>[2x]WGAPTITNDGVSIAKEIELEDPYEKIGAELVKEVAKKTDDVAGDGTTTATVLAQALVREGLRNVAAGANPLGLKRGIEKAVEKVTETLLKGAKEVETKEQIAATAAISAGDQSIGDLIAEAMDKVGNEGVITVEESNTFGLQLELTEGMRFDK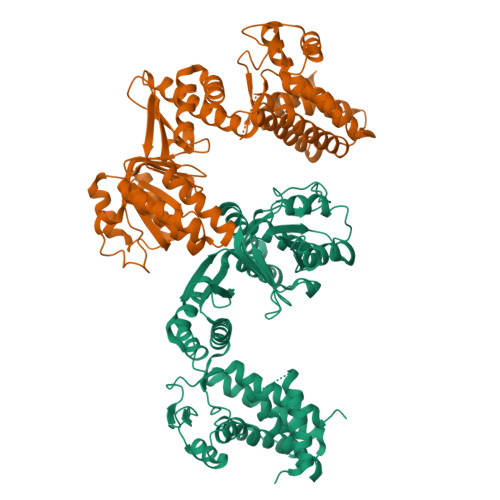GYISGYFVTDPERQEAVLEDPYILLVSSKVSTVKDLLPLLEKVIGAGKPLLIIAEDVEGEALSTLVVNKIRGTFKSVAVKAPGFGDRRKAMLQDMAILTGGQVISEEVGLTLENADLSLLGKARKVVVTKDETTIVEGAGDTDAIAGRVAQIRQEIENSDSDYDREKLQERLAKLAGGVAVIKAGAATEVELKERKHRIEDAVRNAKAAVEEGIVAGGGVTLLQAAPTLDELKLEGDEATGANIVKVALEAPLKQIAFNSGLEPGVVAEKVRNLPAGHGLNAQTGVYEDLLAAGVADPVKVTRSALQNAASIAGLFLTTEAVVADKPEKEKASVPGGGDMGGMDFHHHHHH>GVFTFEDESTSTIAPARLYKALVKDADAIIPKAVEAIQSIETVEGNGGPGTIKKLTLIEGGETKYVLHKIEAVDEANLRYNYSIVGGVGLPDTIEKISFETKLVEGANGGSIGKVTIKIETKGDAQP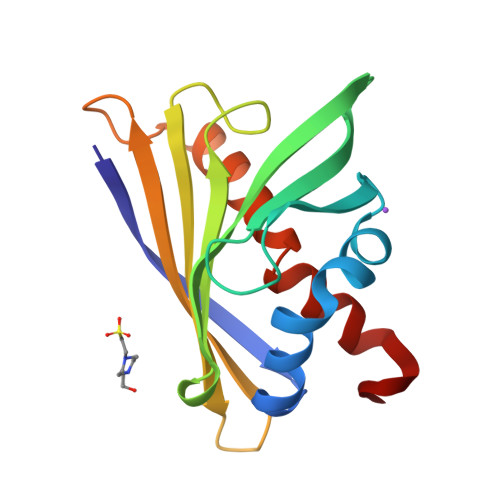NEEEGKAAKARGDAFFKAIENYLSAHPEYN[2x]>[4x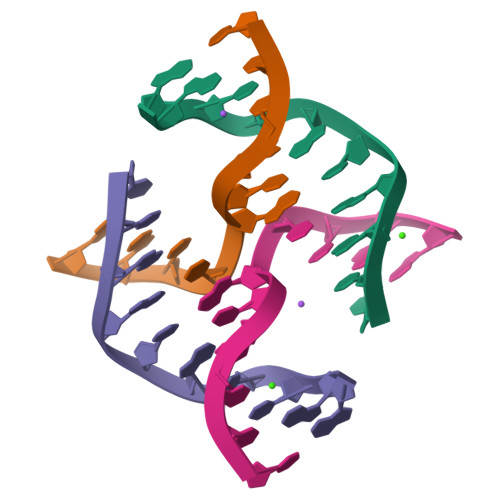]TCGGCGCCGA> MGSSHHHHHHSQDPNSMTTLTRQDLNFGQVVADVLCEFLEVAVHLILYVREVYPVGIFQKRKKYNVPVQMSCHPELNQYIQDTLHCVKPLLEKNDVEKVVVVILDKEHRPVEKFVFEITQPPLLSISSDSLLSHVEQLLRAFILKISVCDAVLDH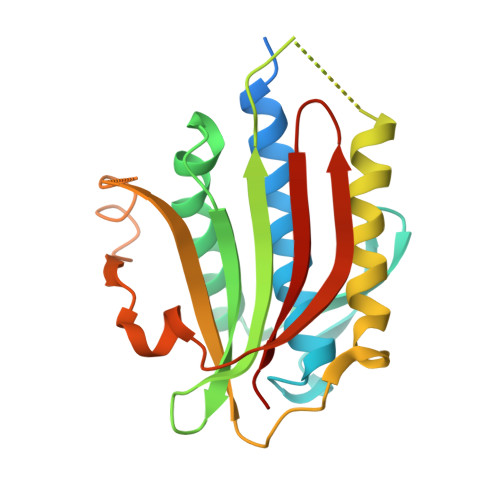NPPGCTFTVLVHTREAATRNMEKIQVIKDFPWILADEQDVHMHDPRLIPLKTMTSDILKMQLYVEERAHKGS>[4x]HPNYKLTYFNMRGRAEIIRYIFAYLDIQYEDHRIEQADWPEIKSTLPFGKIPILEVDGLTLHQSLAIARYLTKNTDL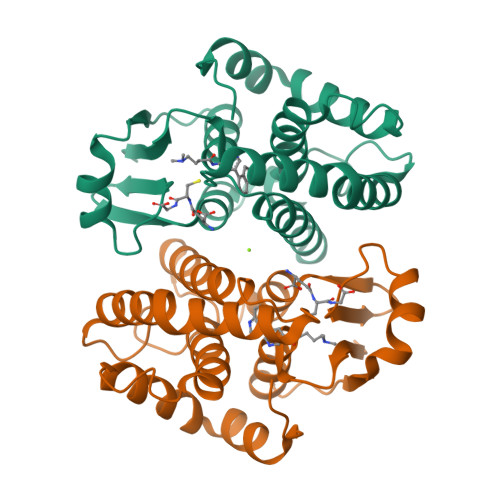AGNTEMEQCHVDAIVDTLDDFMSCFPWAEKKQDVKEQMFNELLTYNAPHLMQDLDTYLGGREWLIGNSVTWADFYWEICSTTLLVFKPDLLDNHPRLVTLRKKVQAIPAVANWIKRRPQTKL>[4x]MGPVWRKHYITYRINNYTPDMNRE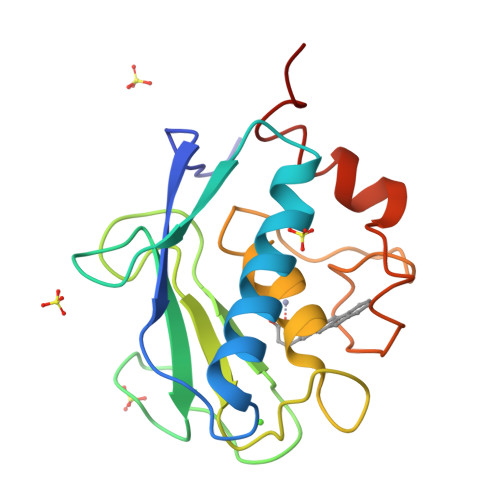DVDYAIRKAFQVWSNVTPLKFSKINTGMADILVVFARGAHGDFHAFDGKGGILAHAFGPGSGIGGDAHFDEDEFWTTHSGGTNLFLTAVHEIGHSLGLGHSSDPKAVMFPTYKYVDINTFRLSADDIRGIQSLYGDPKEN> MKDFQDQVAFITGGASGAGFGQAKVFGQAGAKIVVADVRAEAVEKAVAELEGLGITAHGIVLDIMDREAYARAADEVEAVFGQAPTLLSNTAGVNSFGPIEKTTYDDFDWIIGVNLNGVINGMVTFVPRMIASGRPGHIVTVSSLGGFMGSALAGPYSAAKAASINLMEGYRQGLEKYGIGVSVCTPANIKSNIAEASRLRPAKYGTSGYVENEESIASLHSIHQHGLEPEKLAEAIKKGVEDNALYIIPYPE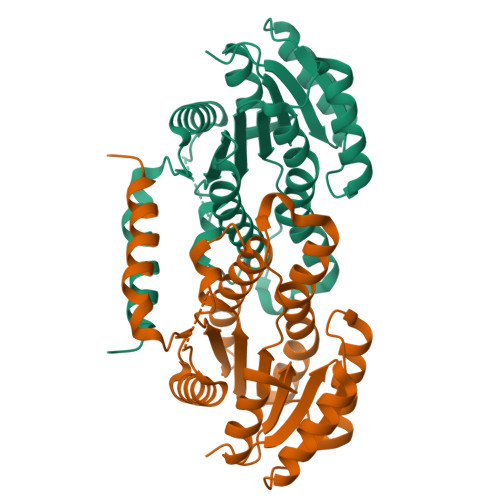VREGLEKHFQAIIDSVAPMESDPEGARQRVEALMAWGRDRTRVFAEGDKKGA> RSTLVHWFRKGLRLHDNPALSHIFTAANAAPGRYFVRPIFILDPGILDWMQVGANRWRFLQQTLEDLDNQLRKLNSRLFVVRGKPAEVFPRIFKSWRVEMLTFETDIEPYSVTRDAAVQKLAKAEGVRVETHCSHTIYNPEALLVIAKNLGKAPITYQKFLGIVEQLKVPKVLGVPEKLKNMPTPPKDEVEQKDSAAYDACCPTMKQLVKRPEELGPNKFPGGETEALRRMEESLKDEIWVARFEKPNTAPNSLEPSTTVLSPYLKFGCLSARLFNQKLKEIIKRQPKHSQPPVSLIGQLMWREFYYTVAAAEPNFD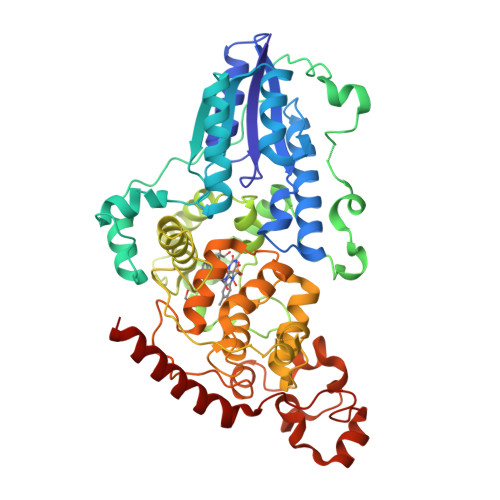RMLGNVYCMQIPWQEAHHPDHLAEEAWTHGRTGYPFIDAIMRQLRQEGWIHHLARHAVACFLTRGDLWISWEEGQRVFEQLLLDQDWALNAGNWMWLSASAFFHQYFRVYSPVAFGKKTDPQGHYIRKYVPELSKYPAGCIYEPWKASLVDQRAYGCVLGTDYPHRIVKHEVVHKENIKRMGAAYKVNREV> GSHMTQFEGFT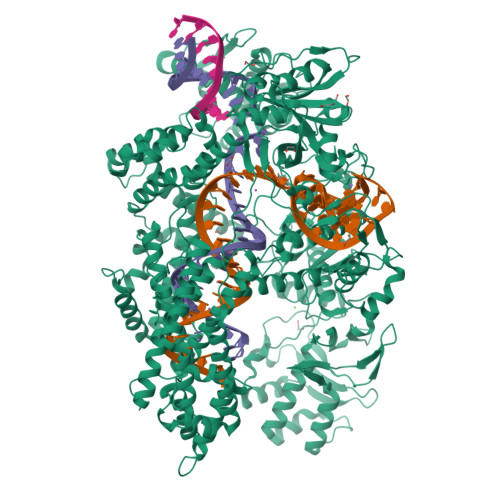NLYQVSKTLRFELIPQGKTLKHIQEQGFIEEDKARNDHYKELKPIIDRIYKTYADQCLQLVQLDWENLSAAIDSYRKEKTEETRNALIEEQATYRNAIHDYFIGRTDNLTDAINKRHAEIYKGLFKAELFNGKVLKQLGTVTTTEHENALLRSFDKFTTYFSGFYENRKNVFSAEDISTAIPHRIVQDNFPKFKENCHIFTRLITAVPSLREHFENVKKAIGIFVSTSIEEVFSFPFYNQLLTQTQIDLYNQLLGGISREAGTEKIKGLNEVLNLAIQKNDETAHIIASLPHRFIPLFKQILSDRNTLSFILEEFKSDEEVIQSFCKYKTLLRNENVLETAEALFNELNSIDLTHIFISHKKLETISSALCDHWDTLRNALYERRISELTGKITKSAKEKVQRSLKHEDINLQEIISAAGKELSEAFKQKTSEILSHAHAALDQPLPTTLKKQEEKEILKSQLDSLLGLYHLLDWFAVDESNEVDPEFSARLTGIKLEMEPSLSFYNKARNYATKKPYSVEKFKLNFQMPTLARGWDVNKEKNNGAILFVKNGLYYLGIMPKQKGRYKALSFEPTEKTSEGFDKMYYDYFPDAAKMIPRCSTQLKAVTAHFQTHTTPILLSNNFIEPLEITKEIYDLNNPEKEPKKFQTAYAKKTGDQKGYREALCKWIDFTRDFLSKYTKTTSIDLSSLRPSSQYKDLGEYYAELNPLLYHISFQRIAEKEIMDAVETGKLYLFQIYNKDFAKGHHGKPNLHTLYWTGLFSPENLAKTSIKLNGQAELFYRPKSRMKRMAHRLGEKMLNKKLKDQKTPIPDTLYQELYDYVNHRLSHDLSDEARALLPNVITKEVSHEIIKDRRFTSDKFFFHVPITLNYQAANSPSKFNQRVNAYLKEHPETPIIGIDRGERNLIYITVIDSTGKILEQRSLNTIQQFDYQKKLDNREKERVAARQAWSVVGTIKDLKQGYLSQVIHEIVDLMIHYQAVVVLENLNFGFKSKRTGIAEKAVYQQFEKMLIDKLNCLVLKDYPAEKVGGVLNPYQLTDQFTSFAKMGTQSGFLFYVPAPYTSKIDPLTGFVDPFVWKTIKNHESRKHFLEGFDFLHYDVKTGDFILHFKMNRNLSFQRGLPGFMPAWDIVFEKNETQFDAKGTPFIAGKRIVPVIENHRFTGRYRDLYPANELIALLEEKGIVFRDGSNILPKLLENDDSHAIDTMVALIRSVLQMRNSNAATGEDYINSPVRDLNGVCFDSRFQNPEWPMDADANGAYHIALKGQLLLNHLKESKDLKLQNGISNQDWLAYIQELRN>[2x]GSHMSDLPLRFPYGRPEFLGLSQDEVEASADHIARPILILKETRRLPWATGYAEVINAGKSTHNEDQASCEVLTVKKKAGAVTSTPNRNSSKRRSSLPNGEGLQLKENSESEGVSCHYWSLFDGHAGSGAAVVASRLLQHHITEQLQDIVDILKNSAVLGSGSTRFFTEKKIPHECLVIGALESAFKEMDLQIERERSSYNISGGCTALIVICLLGKLYVANAGASRAIIIRNGEIIPMSSEFTPETERQRLQYLAFMQPHLLGNEFTHLEFPRRVQRKELGKKMLYRDFNMTGWAYKTIEDEDLKFPLIYGEGKKARVMATIGVTRGLGDHDLKVHDSNIYIKPFLSSAPEVRIYDLSKYDHGSDDVLILATDGLWDVLSNEEVAEAITQFLPNCDPDDPHRYTLAAQDLVMRARGVLKDRGWRISNDRLGSGDDISVYVIPLIHGNKLS

Recent work has shown that the metal‐dependent protein phosphatase PPM1H counteracts LRRK2 by dephosphorylating Rabs. The crystal structure of PPM1H reveals a structurally conserved phosphatase fold that strikingly has evolved a 110‐residue flap domain adjacent to the active site. Cellular assays, crosslinking and 3‐D modelling suggest that the flap domain encodes the docking motif for phosphorylated Rabs. Therefore, PPM1H has acquired a Rab‐specific interaction domain within a conserved phosphatase fold.

We also introduced a D288A mutation (PPM1HDA) that destabilizes a third metal ion (Mg2+/Mn2+) at the active site. Previous studies of PPM1A (D146A) showed that this variant acts as a substrate‐trapping mutant (Debnath et al, 2018). To grow WT crystals and improve diffraction, a “loop deletion” variant of PPM1H (PPM1H‐LD) was designed to eliminate a flexible and non‐conserved loop (188‐226) that was predicted to be distant from the active site. WT and D288A variants of PPM1H (PPM1HWT‐LD, PPM1HDA‐LD) diffracted to 2.5 Å and 2.6 Å resolution, respectively. The variants PPM1HDA, PPM1HWT‐LD, and PPM1HDA‐LD have identical 3‐D structures with two Mg2+ ions at the active site. However, all of the structures are identical with only minor differences arising from flexible loops and the presence or absence of the third metal ion at the active site. The asymmetric unit in all 4 structures is a dimer that is facilitated by interactions between α3 of the flap domains, as well as contacts between the flap domain (residues 356–360) and α2 of the catalytic domain.>[6x]MSQEIRQNEKISYRIEGPFFIIHLMNPDNLNALEGEDYIYLGELLELADRNRDVYFTIIQSSGRFFSSGADFKGIAKAQGDDTNKYPSETSKWVSNFVARNVYVTDA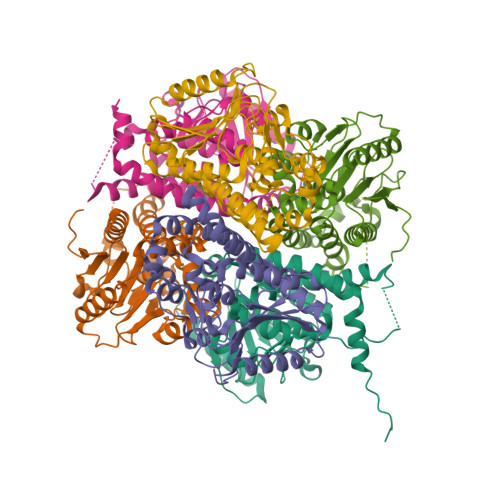FIKHSKVLICCLNGPAIGLSAALVALCDIVYSINDKVYLLYPFANLGLITEGGTTVSLPLKFGTNTTYECLMFNKPFKYDIMCENGFISKNFNMPSSNAEAFNAKVLEELREKVKGLYLPSCLGMKKLLKSNHIDAFNKANSVEVNESLKYWVDGEPLKRFRQLGSKQRKHRL> ATRELDELMASLSDFKFMAQ;> SGRHERDAFDTLFDHAPDKLNVVKKTLITFVNKHLNKLNLEVTELETQFADGVYLVLLMGLLEGYFVPLHSFFLTPDSFEQKVLNVSFAFELMQDGGLEKPKPRPEDIVNCDLKSTLRVLYNLFTKYRNVE

The adaptor protein paxillin contains five conserved leucine-rich (LD) motifs that interact with a variety of focal adhesion proteins, such as α-parvin. α-parvin (Olski et al., 2001), also known as actopaxin or CH-ILKBP (Tu et al., 2001), is part of the ILK signaling complex (Tu et al., 2001), plays an essential role in adhesion-dependent PKB/Act activation (Fukuda et al., 2003) and in the regulation of actin organization (LaLonde et al., 2005) and Rac activation (LaLonde et al., 2005; Zhang et al., 2004). It belongs to the highly conserved parvin family that shares a common architecture composed of a variable N-terminal region followed by two CH domains (Olski et al., 2001). Our results demonstrate that full-length α-parvin contains a single LD binding site, formed by the N-linker helix, helix A, and helix G of the C-terminal type-5 CH domain.

To elucidate the molecular basis for LD recognition by α-parvin-CHC, we cocrystallized α-parvin-CHC with peptides representing the high-affinity ligands LD1, LD2, and LD4. The refined structures include residues 247–372 of α-parvin and paxillin residues 1–14, 141–155, and 262–274 for LD1, LD2, and LD4, respectively. All three LD motifs bind to the same binding site on α-parvin-CHC formed by the N-linker helix, the N-terminal part of helix A and the C-terminal part of helix G, which is consistent with our results from chemical shift mapping. Surprisingly, however, the orientation of LD1 is reversed compared to LD2 and LD4 in the corresponding crystal structures. Despite their antiparallel orientations, however, the binding modes of different LD peptides are very similar. As the result of a slight rotation around the helical axis of the bound peptides, the character and position of side chains facing α-parvin-CHC is largely preserved, the same hydrophobic pockets are occupied, and a similar amount of surface area (∼500 Å2) becomes buried. In addition, two positively charged residues (K260 and R369) of α-parvin-CHC are in close proximity to negatively charged residues of the bound LD peptides. Note that these electrostatic contacts involve the conserved aspartate D+1 of the LD consensus in the case of LD2 and LD4, whereas D+6 and E+8 are utilized in LD1. Consistent with their similar binding modes, all three LD peptides, irrespective of directionality, impose similar conformational changes in the N-terminal region of α-parvin-CHC, whereas the protein core remains virtually unperturbed. In particular, residues 248 to 264, which experience conformational change upon complex formation, are similar in all LD complexes with RMSD-values of 0.28 Å (LD1 versus LD2), 0.23 Å (LD1 versus LD4), and 0.15 Å (LD2 versus LD4) in 16 equivalent Cα−positions.>[2x]SLALHKVIMVGSGGVGKSALTLQFMYDEFVEDYEPTKADSYRKKVVLDGEEVQI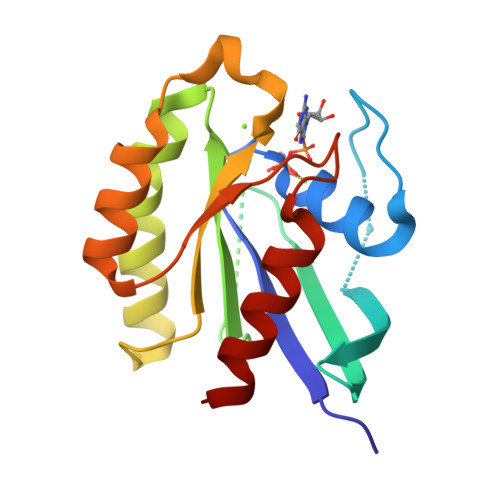DILDTAGQEDYAAIRDNYFRSGEGFLCVFSITEMESFAATADFREQILRVKEDENVPFLLVGNKSDLEDKRQVSVEEAKNRADQWNVNYVETSAKTRANVDKVFFDLMREIRAR> GPLGSMSVAGLKKQFHKATQKVSEKVGGAEGTKLDDDFKEMERKVDVTSRAVMEIMTKTIEYLQPNPASRAKLSMINTMSKIRGQE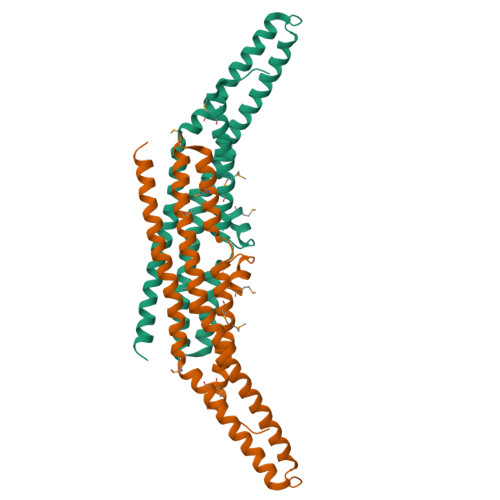KGPGYPQAEALLAEAMLKFGRELGDDCNFGPALGEVGEAMRELSEVKDSLDIEVKQNFIDPLQNLHDKDLREIQHHLKKLEGRRLDFDYKKKRQGKIPDEELRQALEKFDESKEIAESSMFNLLEMDIEQVSQLSALVQAQLEYHKQAVQILQQVTVRLEERIRQA> MGMPVPGTLSVEIPPRYCPLPTARHPDETVLARRTADWIDGFDLELTPQQRARMRGNDAPGFYGRIMPHSPTDRLQLAVDWCTVMFHFDDVHCDEGPATGRAARFADLATRIVRVLEAPDARLEGPGDTMLAPVRDLALRARRWATPAQMRRCAEAHRAWFLAVAWELGHRAARSTPALNDYA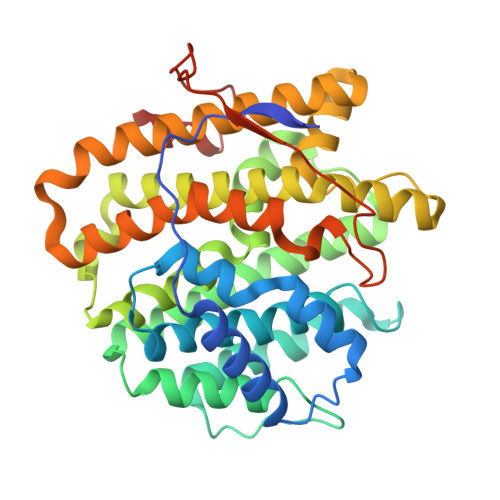HMRQHTAAGAATLAWAEIVDGAEIPDRELSSPEVRALTELAFTTAAFDDDLFSYGKELWVARAEGTAPSGLGLVEILRRENRCGRPEALRAAVCLCNRLTHRFIALRERVLPDASAPLRAYLDHLCHLLPGNLEWGLTADRYRNPDGRTPGAVTTTASRDTDPPADTSPPAIPSIAWWWDPLGGRPATEHHHHHH>[2x]NQIVSGAAWTDTAGNTIQ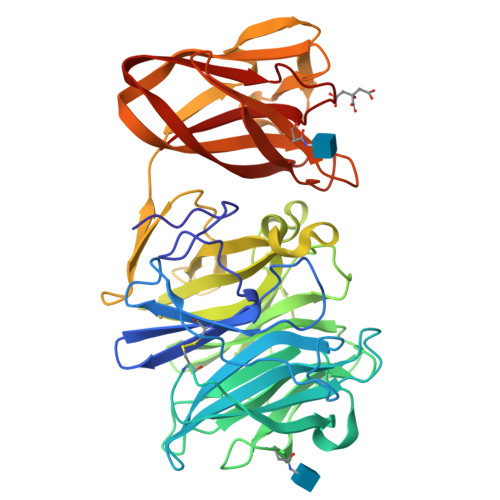AHGAGILQVGSTFYWFGEDKSHNSALFKAVSCYTSSDLVNWSRQNDALSPIAGTMISTSNVVERPKVIFNQKNSEYVMWFHSDSSNYGAAMVGVATAKTPCGPYTYKGSFKPLGADSRDESIFQDDDSAQTAYLLYASDNNQNFKISRLDANYYNVTAQVSVMNGATLEAPGIVKHNGEYFLIASHTSGWAPNPNKWFSASSLAGPWSAQQDIAPSATRTWYSQNAFDLPLGSNAIYMGDRWRPSLLGSSRYIWYPLDFSSGAPQIVHADVWSVNVQAGTYSVASGTSYEAENGQRGGSSTILSGSGFSGGKAVGYLGHGGTVTINNVQSNGGSHWVALYFANGDSTYRNVTVSVNGGPSVLVDQPDSGGGNVVISVPVKLNLNSGENSITFGSGQSNYAADLDKIIVY>[6x]APTKRKGSCPGAAPKKPKEPVQVPKLVIKGGIEVLGVKTGVDSFTEVECFLNPQMGNPDEHQKGLSKSLAAEKQFTDDSPDKEQLPCYSVARIPLPNINEDLTCGNILMWEAVTVKTEVIGVTAMLNLHSGTQKTHENGAGKPIQGSNFHFFAVGGE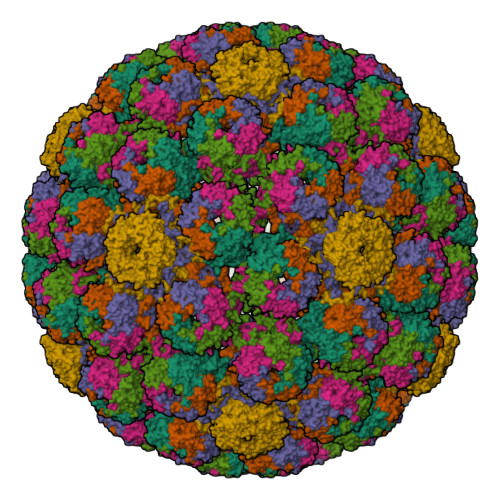PLELQGVLANYRTKYPAQTVTPKNATVDSQQMNTDHKAVLDKDNAYPVECWVPDPSKNENTRYFGTYTGGENVPPVLHITNTATTVLLDEQGVGPLCKADSLYVSAVDICGLFTNTSGTQQWKGLPRYFKITLRKRSVKNPYPISFLLSDLINRRTQRVDGQPMIGMSSQVEEVRVYEDTEELPGDPDMIRYIDEFGQTTTRMQ4,4'-propane-2,2-diylbis(2,6-dibromophenol) | C15 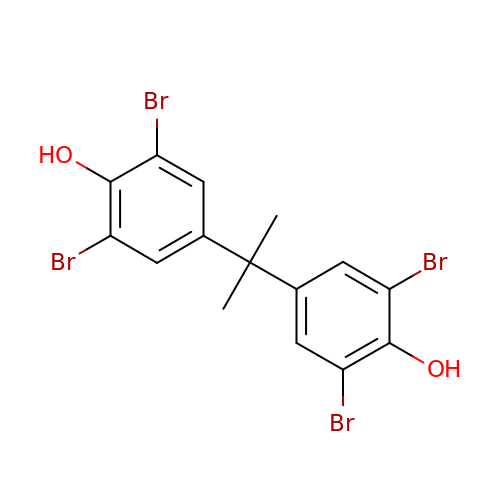H12 Br4 O2 | VEORPZCZECFIRK-UHFFFAOYSA-N> MSTAITRQIVLDTETTGMNQIGAHYEGHKIIEIGAVEVVNRRLTGNNFHVYLKPDRLVDPE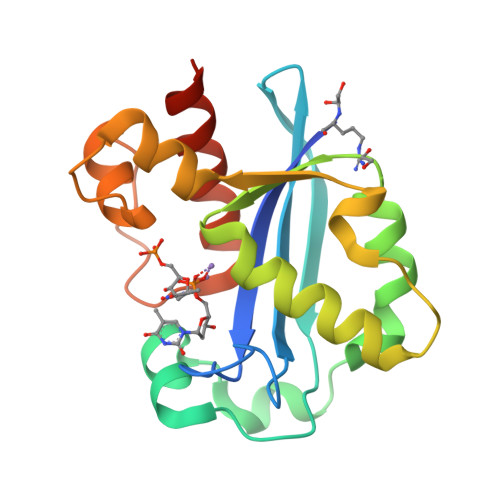AFGVHGIADEFLLDKPTFAEVADEFMDYIRGAELVIHNAAFDIGFMDYEFSLLKRDIPKTNTFCKVTDSLAVARKMFPGKRNSLDALCARYEIDNSKRTLHGALLDAQILAEVYLAMTGGQTSMA> MATNFFIQPITEEAEAYYPPSVITNKRKDLGVDVYCCSDLVLQPGLNIVRLHIKVACEHMGKKCGFKIMARSSMCTHERLLILANGIGLIDPGYVGELMLKIINLGDTPVQIWAKECLVQLVAQGDHVPDHINILKRNQIFPLFAPTPRGEGRFGSTGEAGIMRTHHHHHH

ASFV encodes a dUTP nucleotidohydrolase (dUTPase) (dUTP pyrophosphatase [Dut]; EC 3.6.1.23), called E165R. The enzyme degrades dUTP in the cytoplasm and thus minimizes misincorporation of uracil into viral DNA, which plays an essential role in maintaining the fidelity of genome replication. It is indispensable for reproductive infection of ASFV in swine macrophages, the natural host cell for the virus. We show that E165R is a homotrimer and can specifically hydrolyze dUTP.

The structure of ASFV E165R was solved by molecular replacement, using the structure of P. falciparum dUTPase as a search model, to a resolution of 2.30 Å, with Rwork and Rfree values of 22.2% and 25.5%, respectively. The structure is a closely packed 3-fold symmetric homotrimer, with one E165R trimer in the asymmetric unit. There are 447 visible residues (residues 1 to 149 of the total 165 residues in each subunit) in this structure, which account for 90.3% of the intact protein, and 16 residues at the C terminus of each subunit are missing due to the poor electron density. The E165R protomer in the trimer is mainly composed of β-strands. The 14 β-strands (β1 to β14) form four sheets: β1, β2, β6, β7, and β14 form a parallel/antiparallel mixed sheet, β3, β8, β10, and β13 form an antiparallel sheet, β4 and β12 form another antiparallel sheet, and β5, β9 and β11 form the third antiparallel sheet. One α-helix (α1) and two 310 helices (η1 and η2) appear after β1, β13, and β14, respectively. By comparing the substrate/product binding pockets of apo-E165R and the E165R complex, we found that the binding pocket of apo-E165R is much larger than that of the E165R complex. As calculated by CASTp, the solvent accessible area and volume of the binding pockets in apo-E165R are 249.3 Å2 and 163.2 Å3, respectively. Only their C termini show obvious conformational differences, suggesting high flexibility of the C terminus of E165R.> MAAQGVGPGPGSAAPPGLEAARQKLALRRKKVLSTEEMELYELAQAAGGGIDPDVFKILVDLLKLNVAPLAVFQMLKSMCAGQRLASEPQDPAAVSLPTSSVPETRGRDKGSAALGGVLALAERSNHEGSSQRMPRQPSATRLPKGGGPGKSPTQGST;> MSEFRIHHDVNELLSLLRVHGGDGAEVYIDLLQKNRTPYVTTTVSAHSAKVKIAEFSRTPEDFLKKYDELKSKNTRNLDPLVYLLSKLTEDKETLQYLQQNAKERAELAAAAVGSSTTSINVPAAASKISMQELEELRKQLGSVATGSTLQQSLELKRKMLRDKQNKKNSGQHLPIFPAWVYERPALIGDFLIGAGISTDTALPIVLLRWNLALSPRLKCSGVISAHCNLHLPGTLPLASQESAVVEDLLYVLVGVDGRYVSAQPLAGRQSRTFLVDPNLDLSIRELVHRILPVAASYSAVTRFIEEKSSFEYGQVNHALAAAMRTLVKEHLILVSQLEQLHRQGLLSLQKLWFYIQPAMRTMDILASLATSVDKGECLGGSTLSLLHDRSFSYTGDSQAQELCLYLTKAASAPYFEVLEKWIYRGIIHDPYSEFMVEEHELRKERIQEDYNDKYWDQRYTIVQQQIPSFLQKMADKILSTGKYLNVVRECGHDVTCPVAKEIIYTLKERAYVEQIEKAFNYASKVLLDFLMEEKELVAHLRSIKRYFLMDQGDFFVHFMDLAEEELRKPVEDITPPRLEALLELALRMSTANTDPFKDDLKIDLMPHDLITQLLRVLAIETKQEKAMAHADPTELALSGLEAFSFDYIVKWPLSLIINRKALTRYQMLFRHMFYCKHVERQLCSVWISNKTAKQHSLHSAQWFAGAFTLRQRMLNFVQNIQYYMMFEVMEPTWHILEKNLKSASNIDDVLGHHTGFLDTCLKDCMLTNPELLKVFSKLMSVCVMFTNCMQKFTQSMKLDGELGGQTLEHSTVLGLPAGAEERARKELARKHLAEHADTVQLVSGFEATINKFDKNFSAHLLDLLARLSIYSTSDCEHGMASVISRLDFNGFYTERLERLSAERSQKATPQVPVLRGPPAPAPRVAVTAQ;>MMDLVLEEDVTVPGTLSGCSGLVPSVPDDLDGINPNAGLGNGLLPNVSEETVSPTRARNMKDFENQITELKKENFNLKLRIYFLEERMQQEFHGPTEHIYKTNIELKVEVESLKRELQEREQLLIKASKAVESLAEAGGSEIQRVKEDARKKVQQVEDLLTKRILLLEKDVTAAQAELEKAFAGTETEKALRLRLESKLSEMKKMHEGDLAMALVLDEKDRLIEELKLSLKSKEALIQCLKEEKSQMACPDENVSSGELRGLCAAPREEKERETEAAQMEHQKERNSFQERIQALEEDLREKEREIATEKKNSLKRDKAIQGLTMALKSKEKKVEELNSEIEKLSAAFAKAREALQKAQTQEFQGSEDYETALSGKEALSAALRSQNLTKSTENHRLRRSIKKITQELSDLQQERERLEKDLEEAHREKSKGDCTIRDLRNEVEKLRNEVNEREKAMENRYKSL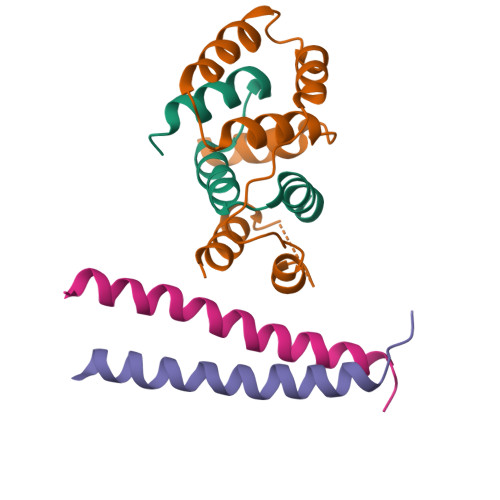LSESNKKLHNQEQVIKHLTESTNQKDVLLQKFNEKDLEVIQQNCYLMAAEDLELRSEGLITEKCSSQQPPGSKTIFSKEKKQSSDYEELIQVLKKEQDIYTHLVKSLQESDSINNLQAELNKIFALRKQLEQDVLSYQNLRKTLEEQISEIRRREEESFSLYSDQTFYLSICLEENNRFQVEHFSQEELKKKVSDLIQLVKELYTDNQHLKKTIFDLSCMGFQGNGFPDRLASTEQTELLASKEDEDTIKIGEDDEINFLSDQHLQQSNEIMKDLSKGGCKNGYLRHTESKISDCDGAHAPGCLEEGAFINLLAPLFNEKATLLLESRPDLLKVVRELLLGQLFLTEQEVSGEHLDGKTEKTPKQKGELVHFVQTNSFSKPHDELKLSCEAQLVKAGEVPKVGLKDASVQTVATEGDLLRFKHEATREAWEEKPINTALSAEHRPENLHGVPGWQAALLSLPGITNREAKKSRLPILIKPSRSLGNMYRLPATQEVVTQLQSQILELQGELKEFKTCNKQLHQKLILAEAVMEGRPTPDKTLLNAQPPVGAAYQDSPGEQKGIKTTSSVWRDKEMDSDQQRSYEIDSEICPPDDLASLPSCKENPEDVLSPTSVATYLSSKSQPSAKVSVMGTDQSESINTSNETEYLKQKIHDLETELEGYQNFIFQLQKHSQCSEAIITVLCGTEGAQDGLSKPKNGSDGEEMTFSSLHQVRYVKHVKILGPLAPEMIDSRVLENLKQQLEEQEYKLQKEQNLNMQLFSEIHNLQNKFRDLSPPRYDSLVQSQARELSLQRQQIKDGHGICVISRQHMNTMIKAFEELLQASDVDYCVAEGFQEQLNQCAELLEKLEKLFLNGKSVGVEMNTQNELMERIEEDNLTYQHLLPESPEPSASHALSDYETSEKSFFSRDQKQDNETEKTSVMVNSFSQDLLMEHIQEIRTLRKRLEESIKTNEKLRKQLERQGSEFVQGSTSIFASGSELHSSLTSEIHFLRKQNQALNAMLIKGSRDKQKENDKLRESLSRKTVSLEHLQREYASVKEENERLQKEGSEKERHNQQLIQEVRCSGQELSRVQEELKLRQQLLSQNDKLLQSLRVELKAYEKLDEEHRRLREASGEGWKGQDPFRDLHSLLMEIQALRLQLERSIETSSTLQSRLKEQLARGAEKAQEGALTLAVQAVSIPEVPLQPDKHDGDKYPMESDNSFDLFDSSQAVTPKSVSETPPLSGNDTDSLSCDSGSSATSTPCVSRLVTGHHLWASKNGRHVLGLIEDYEALLKQISQGQRLLAEMDIQTQEAPSSTSQELGTKGPHPAPLSKFVSSVSTAKLTLEEAYRRLKLLWRVSLPEDGQCPLHCEQIGEMKAEVTKLHKKLFEQEKKLQNTMKLLQLSKRQEKVIFDQLVVTHKILRKARGNLELRPGGAHPGTCSPSRPGS[2x]> NVLTVYSPYQSNLIRPILNEFEKQEHVKIEIKHGSTQVLLSNLHNEDFSERGDVFMGGVLSETIDHPEDFVPYQDTSVTQQLEDYRSNNKYVTSFLLMPTVIVVNSDLQGDIKIRGYQDLLQPILKGKIAYSNPNTTTTGYQHMRAIYSMHHRVSDVHQFQNHAMQLSKTSKVIEDVAKGKYYAGLSYEQDARTWKNKGYPVSIVYPIEGTMLNVDGIALVKNAHPHPKRKKLVQYLTSRSVQQRLVAEFDA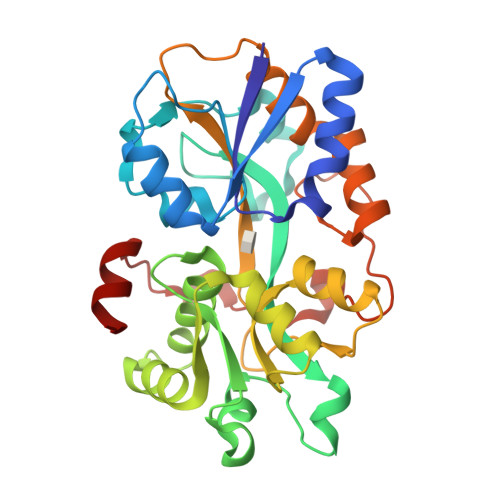KSIRKDVSEQSDQSIENLKNIPLIPKSKLPDIPHHKFLEMIQ>[2x]MTADELVFFVNGKKVVEKNADPETTLLVYLRRKLGLCGTKLGCGEGGCGACTVMISKYDRLQNKIVHFSVNACLAPICSLHHVAVTTVEGIGN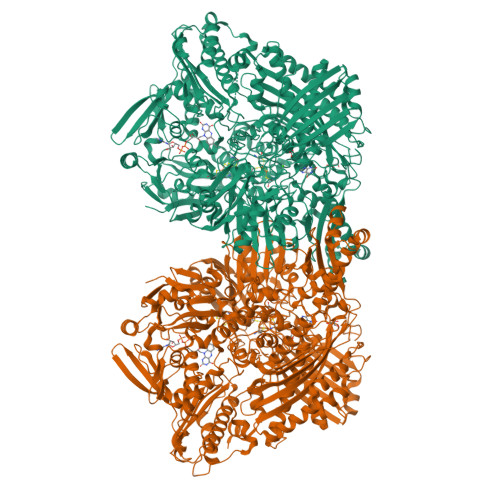TQKLHPVQERIARSHGSQCGFCTPGIVMSMYTLLRNQPEPTVEEIENAFQGNLCRCTGYRPILQGFRTFAKDGGCCGGSGNNPNCCMNQTKDQTVSLSPSLFNPEDFKPLDPTQEPIFPPELLRLKDTPQKKLRFEGERVTWIQASTMEELLDLKAQHPDAKLVVGNTEIGIEMKFKNMLFPLIVCPAWIPELNSVVHGPEGISFGASCPLSLVESVLAEEIAKLPEQKTEVFRGVMEQLRWFAGKQVKSVASIGGNIITASPISDLNPVFMASGAKLTLVSRGTRRTVRMDHTFFPGYRKTLLRPEEILLSIEIPYSKEGEFFSAFKQASRREADIAKVTSGMRVLFKPGTIEVQELSLCFGGMADRTISALKTTPKQLSKSWNEELLQSVCAGLAEELQLAPDAPGGMVEFRRTLTLSFFFKFYLTVLQKLGRADLEDMCGKLDPTFASATLLFQKDPPANVQLFQEVPKDQSEEDMVGRPLPHLAANMQASGEAVYCDDIPRYENELSLRLVTSTRAHAKITSIDTSEAKKVPGFVCFLTAEDVPNSNATGLFNDETVFAKDEVTCVGHIIGAVVADTPEHAQRAARGVKITYEDLPAIITIQDAINNNSFYGSEIKIEKGDLKKGFSEADNVVSGELYIGGQEHFYLETNCTIAVPKGEAGEMELFVSTQNTMKTQSFVAKMLGVPDNRIVVRVKRMGGGFGGKETRSTVVSTALALAAHKTGRPVRCMLDRDEDMLITGGRHPFLAKYKVGFMKTGTVVALEVAHFSNGGNTEDLSRSIMERALFHMDNAYKIPNIRGTGRICKTNLPSNTAFRGFGGPQGMLIAEYWMSEVAITCGLPAEEVRRKNMYKEGDLTHFNQKLEGFTLPRCWDECIASSQYLARKREVEKFNRENCWKKRGLCIIPTKFGISFTLPFLNQGGALVHVYTDGSVLLTHGGTEMGQGLHTKMVQVASRALKIPTSKIHISETSTNTVPNTSPTAASASADLNGQGVYEACQTILKRLEPFKKKKPTGPWEAWVMDAYTSAVSLSATGFYKTPNLGYSFETNSGNPFHYFSYGVACSEVEIDCLTGDHKNLRTDIVMDVGSSLNPAIDIGQVEGAFVQGLGLFTMEELHYSPEGSLHTRGPSTYKIPAFGSIPIEFRVSLLRDCPNKRAIYASKAVGEPPLFLASSIFFAIKDAIRAARAQHGDNAKQLFQLDSPATPEKIRNACVDQFTTLCVTGVPENCKSWSVRI5-fluoro-2-({[(3M)-3-(1H-imidazol-2-yl)pyridin-2-yl]amino}methyl)phenol | C15 H13 F N4 O | 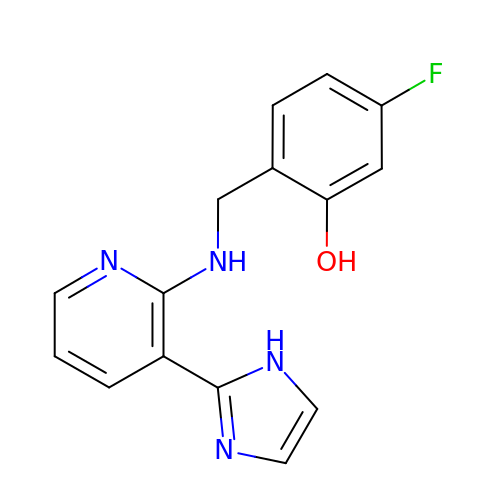MFPPUJHTLAJSCS-UHFFFAOYSA-N>MELRVGNRYRLGRKIGSGSFGDIYLGTDIAAGEEVAIKLECVKTKHPQLHIESKIYKMMQGGVGIPTIRWCGAEGDYNVMVMELLGPSLEDLFNFCSRKFSLKTVLLLADQMISRIEYIHSKNFIHRDVKPDNFLMGLGKKGNLVYIIDFGLAKKYRDARTHQHIPYRENENLTGTARYASINTHLGIEQSRRDDLESLGYVLMYFNLGSLPWQGLKAATKRQKYERISEKKMSTPIEVLCKGYPSEFATYLNFCRSLRFDDKPDYSYLRQLFRNLFHRQG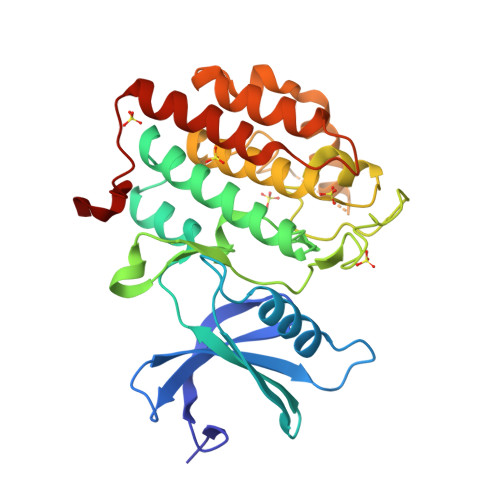FSYDYVFDWNMLK[2x]>[4x]GAMGSNIESTLNSVASVKDLANEASKYEIILQKGINQVGLKQYTQVVHKLDDMLEDIQSGQANREENSEFHGILTHLEQLIKRSEAQLRVYFISILNSIKPFDPQINITKKMPFPYYEDQQLGALSWILDYFHGNSEGSIIQDILVGERSKLILKCMAFLEPFAKEISTAKNAPYEKGSSGMNSYTEALLGFIANEKSLVDDLYSQYTESKPHVLSQILSPLISAYAKLFGANLKIVRSNLENFGFFSFELVESINDVKKSLRGKELQNYNLLQDCTQEVRQVTQSLFRDAIDRIIKKANSISTIPSNNGVTEATVDTMSRLRKFSEYKNGCLGAMDNITRENWLPSNYKEKEYTLQNEALNWEDHNVLLSCFISDCIDT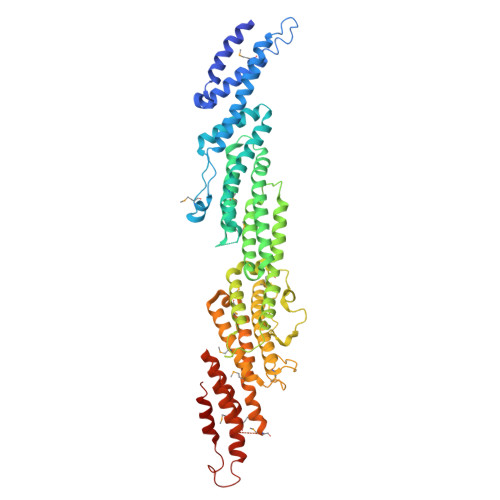LAVNLERKAQIALMPNQEPDVANPNSSKNKHKQRIGFFILMNLTLVEQIVEKSELNLMLAGEGHSRLERLKKRYISYMVSDWRDLTANLMDSVFIDSSGKKSKDKEQIKEKFRKFNEGFEDLVSKTKQYKLSDPSLKVTLKSEIISLVMPMYERFYSRYKDSFKNPRKHIKYTPDELTTVLNQLVR> GSHMVKQLKWRTVNPEETKAIAKLTAAFAKPGDVLTLEGDLGAGKTTFTKGFAEGLGITRIVNSPTFTIIKEYNDGVLPLYHMDVYRMEDESEDLGLDEYFHGQGVCLVEWAHLIEEQLPQERLQIVIKRAGDDEREITFTAVGNRYEML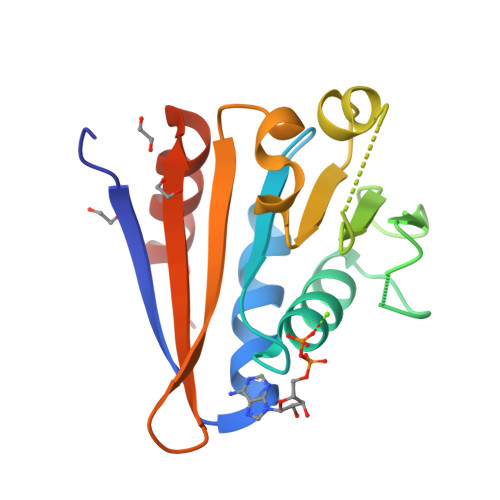CEELSRHDNISN>MTTETLVSGTTPVSDNANLKQHLTTPTQEGQTLRDSVEKALHNYFAHLEGQPVTDVYNMVLCEVEAPLLETVMNHVKGNQTKASELLGLNRGTLR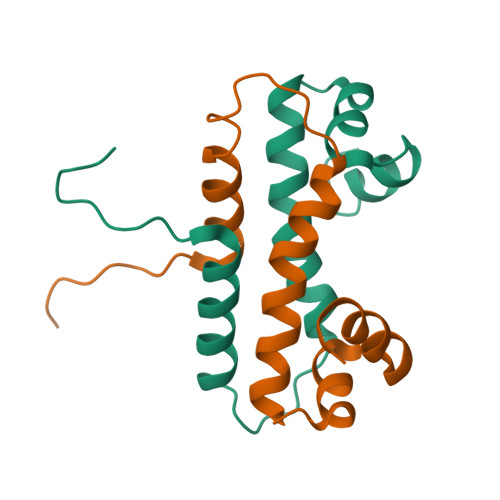KKLKQYDLL[4x]> APVWGCASTRGRSAEMEDASAAVPRFADVPVRLLASRRDLDALGLDADALRLPAHLFGVFDGHGGAEVANYCRERIHVVLSAALARLGKNLGEMGEVDMKEHW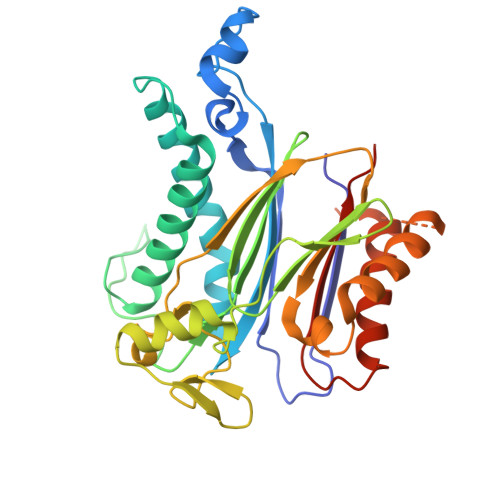DDVFTKCFQRVDDEVSGRVTRVVNGGGEVRSEPVTAENVGSTAVVALVCSSHVVVANCGDSRIVLCRGKEPVALSIDHKPDRKDERARIEAQGGKVIQWNGYRVSGWLAMSRSIGDRYLKPFVIPKPEVMVVPRAKDDDCLILASDGLWDVVSNEEACKVARRQILLWHKNNGAASPLSDEGEGSTDPAAQAAADYLMRLALKKGSEDNITVIVVDLKPRKKLKN> VMATGCFVGARNASEPRLGSSSIAASRTAPAYLREAQVLYEGSTDG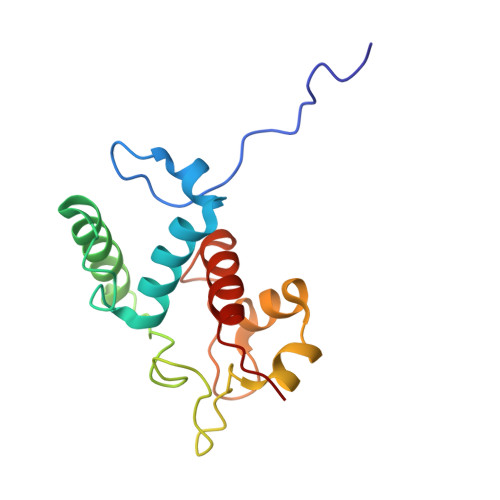LPKDTPADEIAHYKAMLAELQTRNYAACAGCHQVNGGGNKAINATNFQDAGWQANNSSPGMVTSIVNGKGKVMPAYKDKLTLQQINYLVEYIRRFEKKR2',3'-DEHYDRO-2',3'-DEOXY-THYMIDINE 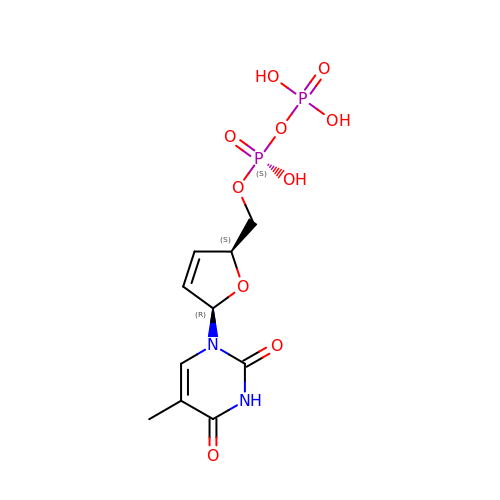5'-DIPHOSPHATE | C10 H14 N2 O10 P2 | LXCAIISEDMYORY-JGVFFNPUSA-N>MAHCTEYMNAPKKLPADVAEELATTAQKLVQAGKGILAADESTQTIKKRFDNIKLENTIENRASYRDLLFGTKGLGKFISGAILFEETLFQKNEAGVPMVNLLHNENIIPGIKVDKGLVNIPCTDEEKSTQGLDGLAERCKEYYKAGARFAKWRTVLVIDTAKGKPTDLSIHETAWGLARYASICQQNRLVPIVEPEILADGPHSIEVCAVVTQKVLSCVFKALQENGVLLEGALLKPNMVTAGYECTAKTTTQDVGFLTVRTLRRTVPPALPGVVFLSGGQSEEEASVNLNSINALGPHPWAL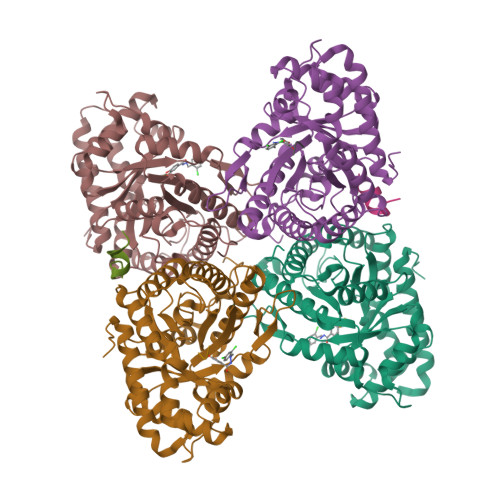TFSYGRALQASVLNTWQGKKENVAKAREVLLQRAEANSLATYGKYKGGAGGENAGASLYEKKYVY[4x];> AASLYEKKAA;> AAASLYEKKAA;>[4x]DWN> MTVKVCVCGGGNGAHTLSGLAASRDGVEVRVL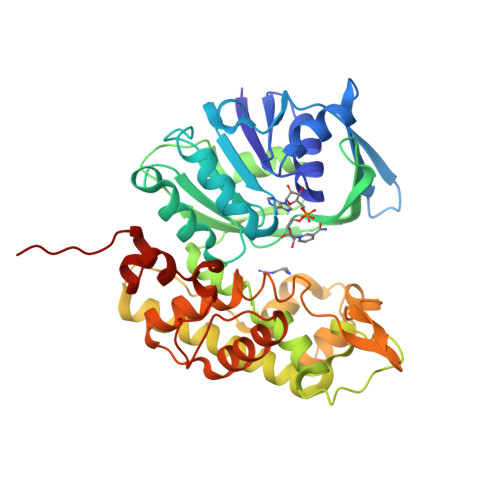TLFADEAERWTKALGADELTVIVNEKDGTQTEVKSRPKVITKDPEIAISGADVVILTVPAFAHEGYFQAMAPYVQDSALIVGLPSQAGFEFQCRDILGDKAAAVSMMSFETLPWACRIKEFGRKVEVLGTKSVLAASLIKGTAKTVDPLSTLQMLHGAEPVFRLAKHFLEMLIMSYSFVHPAILFGRWGSWDGKPVPEAPLFYQGIDQATADMLTACSNECKDVANAIMAACPGNDLSDDKDIYQWYLEYYHEDIQDDHDLYHAITTNKSYKGLVHPVKAVDAGVAPDFGNRYLTEDIPMGMIVFKGVAIAAGVAIPSNDKLIMWAQEKIGKEYLVDGALTGKDVATTRCPQRYGFNTLDAILTGKKHHHHH> AGGCGCAUUUGAACUGUAUUGUACGCCUUGCAUAAAGCAAAAG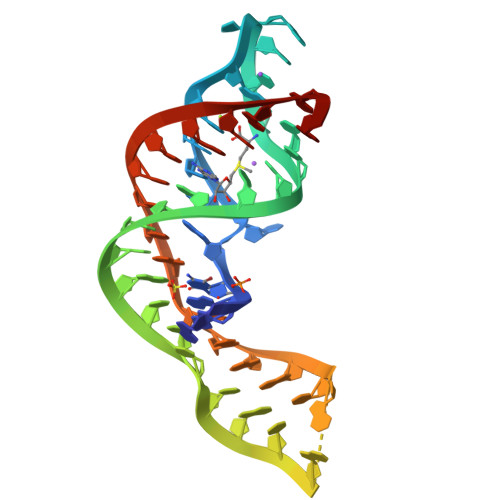UACUAAAAAA>MGSSHHHHHHSSGLVPRGSEHLKNISPIDGRYKKACGELSAFFSEHALIKHRIIVEVRWLLFLNEEELFFEKVTDHSVEVLNQIATNITDSDIARVKAIEEETNHDVKAVEYFVKEKLKNSKREDLLKIKEYVHYLCTSEDINNVAYATCLKACLNDVVIPCLEKIMLKLKDLAVEYSHVPLLSRTHGQPASSTTFGKEMANFYARIHHHVGVIRRVKVCAKFNGAVGNFNAHKVASKDTDWVNTIGLFLKKHFNLTYSIYCTQIQDHDYICELCDGLARANGTLIDLCVDIWLYISNNLLKLKVKEKEVGSSTMPHKVNPIDFENAEGNLHIANAFFKLFSSKLPTSRLQRDLSDSTVLRNIGSSLAYCLIAYKSVLKGLNKIDIDRRNLEEELNQNWSTLAEPIQIV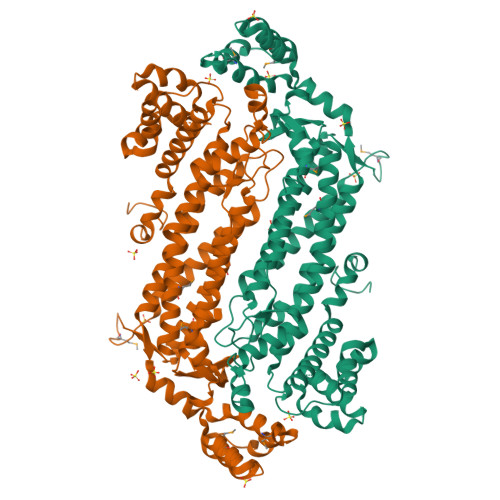MKRHNYVDAYEELKQFTRGKVIDQKIMQEFIKTKCAFLPQDVVDQLLELTPATYTGYADYLAKNVERLSGERD[2x]> HHHHHHHHHHEQKLISEEDLDYKDDDDKMESEMLQSPLLGLGEEDEADLTDWNLPLAFMKKRHCEKIEGSKSLAQSWRMKDRMKTVSVALVLCLNVGVDPPDVVKTTPCARLECWIDPLSMGPQKALETIGANLQKQYENWQPRARYKQSLDPTVDEVKKLCTSLRRNAKEERVLFHYNGHGVPRPTVNGEVWVFNKNYTQYIPLSIYDLQTWMGSPSIFVYDCSNAGLIVKSFKQFALQREQELEVAAINPNHPLAQMPLPPSMKNCIQLAACEATELLPMIPDLPADLFTSCLTTPIKIALRWFCMQKCVSLVPGVTLDLIEKIPGRLNDRRTPLGELNWIFTAITDTIAWNVLPRDLFQKLFRQDLLVASLFRNFLLAERIMRSYNCTPVSSPRLPPTYMHAMWQAWDLAVDICLSQLPTIIEEGTAFRHSPFFAEQLTAFQVWLTMGVENRNPPEQLPIVLQVLLSQVHRLRALDLLGRFLDLGPWAVSLALSVGIFPYVLKLLQSSARELRPLLVFIWAKILAVDSSCQADLVKDNGHKYFLSVLADPYMPAEHRTMTAFILAVIVNSYHTGQEACLQGNLIAICLEQLNDPHPLLRQWVAICLGRIWQNFDSARWCGVRDSAHEKLYSLLSDPIPEVRCAAVFALGTFVGNSAERTDHSTTIDHNVAMMLAQLVSDGSPMVRKELVV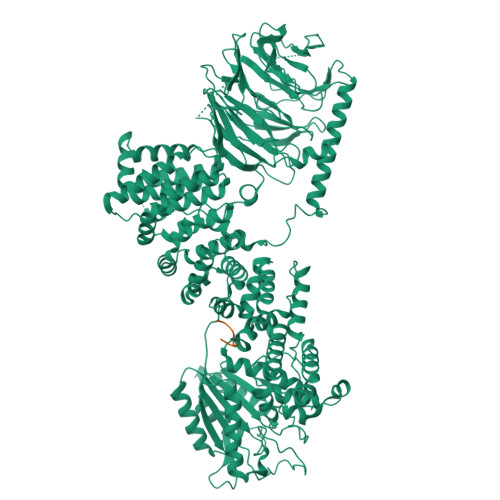ALSHLVVQYESNFCTVALQFIEEEKNYALPSPATTEGGSLTPVRDSPCTPRLRSVSSYGNIRAVATARSLNKSLQNLSLTEESGGAVAFSPGNLSTSSSASSTLGSPENEEHILSFETIDKMRRASSYSSLNSLIGVSFNSVYTQIWRVLLHLAADPYPEVSDVAMKVLNSIAYKATVNARPQRVLDTSSLTQSAPASPTNKGVHIHQAGGSPPASSTSSSSLTNDVAKQPVSRDLPSGRPGTTGPAGAQYTPHSHQFPRTRKMFDKGPEQTADDADDAAGHKSFISATVQTGFCDWSARYFAQPVMKIPEEHDLESQIRKEREWRFLRNSRVRRQAQQVIQKGITRLDDQIFLNRNPGVPSVVKFHPFTPCIAVADKDSICFWDWEKGEKLDYFHNGNPRYTRVTAMEYLNGQDCSLLLTATDDGAIRVWKNFADLEKNPEMVTAWQGLSDMLPTTRGAGMVVDWEQETGLLMSSGDVRIVRIWDTDREMKVQDIPTGADSCVTSLSCDSHRSLIVAGLGDGSIRVYDRRMALSECRVMTYREHTAWVVKASLQKRPDGHIVSVSVNGDVRIFDPRMPESVNVLQIVKGLTALDIHPQADLIACGSVNQFTAIYNSSGELINNIKYYDGFMGQRVGAISCLAFHPHWPHLAVGSNDYYISVYSVEKRVR;> MMNRFRKWLYKPKRSDPQLLARFYYADEELNQVAAELDSLDGRKDPQRCTLLVSQFRSCQDNVLNIINQIMDECIPQDRAPRDFCVKFPEEIRHDNLAGQLWFGAECLAAGSIIMNRELESMAMRPLAKELTRSLEDVRGALRDQALRDLNTYTEKMREALRHFDVLFAEFELSYVSAMVPVKSPREYYVQQEVIVLFCETVERALDFGYLTQDMIDDYEPALMFSIPRLAIVCGLVVYADGPLNLDRKVEDMSELFRPFHTLLRKIRDLLQTLTEEELHTLERNLCISQDVEFPIRADVQGPAALAPALSAPLPPEGPLSAKAKDPDAELACSMQYDDQELEQLSRMVHRAGDEMSSLLSPPIACQSPAHRPGAEGSPGGEASPGRPRLRSGSDEEERVFFMDDVEGTAEALARPESPAGPFGWAGSTWADPQEKGQGGPGGAAGISLPASEKEEDLSNNNLEAEGTDGASLAGTSSCSCLDSRLHLDGWEVGADDAETAEMIAHRTGGMKLSATVIFNPKSPTSLDSAVATQEAASEPVAEGMDGGPHKLSTGATNCLLHSCVCCGSCGDSREDVVERLREKCSPGGVIGASYAAGLAKASDRAPERQEEAPPPSEDASNGREPKAPTSDKCLPHTSGSQVDTASGLQGEAGVAGQQEPEARELHAGSPSAHEAPQALSGSSSSTAGSCSSDKMGPEAAPAATHAAPQATREKIRSRFHGSHDLIHRLFVCISGVADQLQTNYASDLRSILKTLFEVMATKPETDDKEKLRKVTQTLRSAALEDCALCQETLSSSELAAKTRDGDFEDPPEWVPDEACGFCTACKAPFTVIRRKHHCRSCGKIFCSRCSSHSAPLPRYGQVKPVRVCTHCYMFHVTPFYSDKAGL2-(carbamoylamino)-5-(4-fluorophenyl)thiophene-3-carboxamide 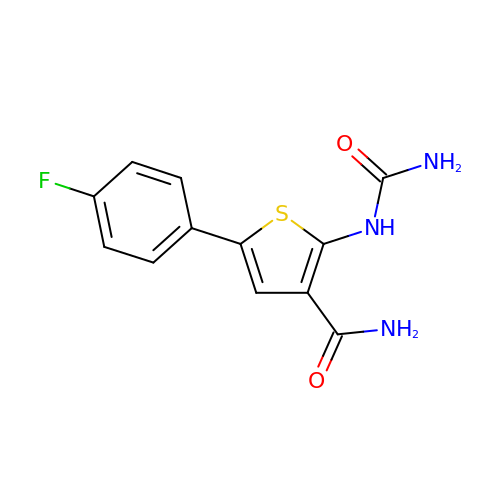| C12 H10 F N3 O2 S | SAYGKHKXGCPTLX-UHFFFAOYSA-N> MIELVIVSRLLEYPDAALWQHQQEMFEAIAASKNLPKEDAH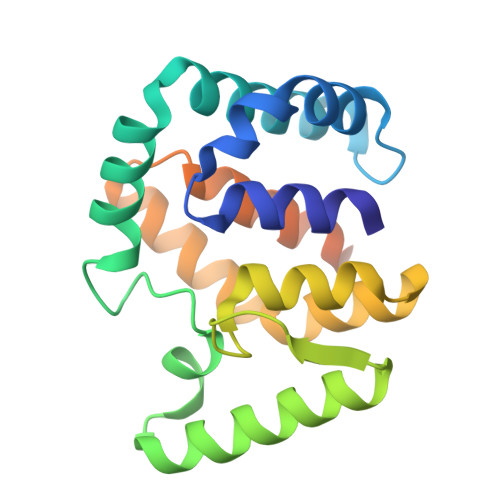ALGIFLRDLTTMDPLDAQAQYSELFDRGRATSLLLFEHVHGESRDRGQAMVDLLAQYEQHGLQLNSRELPDHLPLYLEYLAQLPQSEAVEGLKDIAPILALLSARLQQRESRYAVLFDLLLKLANTAIDSDKVAEKIADEARPGAHHHHHH> MYITKIVIQGFKSYKDYTVIEPLSPHHNVIVGRNGSGKSNFFAAIRFVLSDAYTHLSREERQALLHEGPGATVMSAYVEVTFANADNRFPTGKSEVVLRRTIGLKKDEYSLDKKTVSKTEVINLLESAGFSRSNPYYIVPQGRVTSLTNAKDSERLELLKEVAGTQIYENRRAESNKIMDETIQKSEKIDELLQYIEERLRELEEEKNDLAVYHKKDNERRCLEYAIYSREHDEINSVLDALEQDRIAALERNDDDSGAFIQREERIERIKAEITELNHSLELLRVEKQQNDEDYTNIMKSKVALELQSSQLSRQIEFSKKDESSKLNILSELESKISEKENELSEILPKYNAIVSEADDLNKRIMLLKNQKQSLLDKQSRTSQFTTKKERDEWIRNQLLQINRNINSTKENSDYLKTEYDEMENELKAKLSRKKEIEISLESQGDRMSQLLANITSINERKENLTDKRKSLWREEAKLKSSIENVKDDLSRSEKALGTTMDRNTSNGIRAVKDIAERLKLEGYYGPLCELFKVDNRFKVAVEATAGNSLFHIVVDNDETATQILDVIYKENAGRVTFMPLNKLRPKAVTYPDASDALPLIQYLEFDPKFDAAIKQVFSKTIVCPSIETASQYARSHQLNGITLSGDRSDKKGALTAGYRDYRNSRLDAIKNVKTYQIKFSDLQESLEKCRSEIESFDQKITACLDDLQKAQLSLKQFERDHIPLKDELVTITGETTDLQESMHHKSRMLELVVLELHTLEQQANDLKSELSSEMDELDPKDVEALKSLSGQIENLSHEFDAIIKERAHIEARKTALEYELNTNLYLRRNPLKAEIGSDNRIDESELNSVKRSLLKYENKLQIIKSSSSGLEEQMQRINSEISDKRNELESLEELQHEVATRIEQDAKINERNAAKRSLLLARKKECNEKIKSLGVLPEEAFIKYVSTSSNAIVKKLHKINEALKDYGSVNKKAYEQFNNFTKQRDSLLARREELRRSQESISELTTV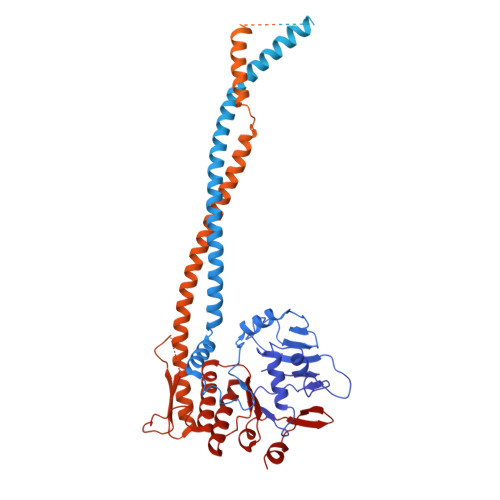LDQRKDEAIERTFKQVAKSFSEIFVKLVPAGRGELVMNRRSELSQSIEQDISMDIDTPSQKSSIDNYTGISIRVSFNSKDDEQLNINQLSGGQKSLCALTLIFAIQRCDPAPFNILDECDANLDAQYRSAIAAMVKEMSKTSQFICTTFRPEMVKVADNFYGVMFNHKVSTVESISKEEAMAFVEG Members of the DAPK family are generally involved in both apoptotic and autophagy pathways and share significant overall sequence similarity with myosin light chain-related kinases and triple functional domain protein-related kinases (Temmerman et al., 2013). DAPK1 and DAPK2 bind Ca2+/CaM through a closely related ARD, which is inhibited by phosphorylation of an identical ARD residue Ser308 in both kinases (Shani et al., 2001, Shohat et al., 2001). They also contain a basic loop (BL) in the kinase N lobe next to the kinase active site, which has been identified as a DAPK-family-specific signature motif (Tereshko et al., 2001). We found an identical type of dimer arrangement in all three kinases that involves the BL of the CD. In terms of functional implications, CD dimerization in hDAPK1, hDAPK2, and hDAPK3 is likely to inhibit catalytic activity by directly occluding the kinase active site.

To explore the molecular mechanisms involved in human DAPK regulation, we expressed and purified truncated versions of hDAPK1, hDAPK2, and hDAPK3. Both the hDAPK1 and hDAPK2 constructs encompass the CD and ARD segments. All three kinases were crystallized and the resulting structures were refined to a resolution of 2.0 Å (hDAPK1), 1.47 Å (hDAPK2), and 3.1 Å (hDAPK3). The hDAPK2 crystal contained two of these dimers per asymmetric unit, referred to as chains A/B and C/D, which provided an additional assessment of experimental error (details described in the legend). We addressed this question using hDAPK2, as its high-resolution structure provides the most accurate data on dimer interface interactions. The second main dimer interface is formed from positively charged residues on the DAPK signature BL segment, which belongs to the most mobile areas in the DAPK structures. In DAPK2, the main residues that contribute to the polar interactions are Arg47, Arg50, and Arg53 as well as the active-site residue Glu100 and Asp220 from the loop preceding helix αG. By contrast, in the DAPK2 structure, Glu182 is blocked by an interaction with Arg303 from the ARD, which acts as a pseudosubstrate. DAPK2 comprises an additional C-terminal tail segment that is predicted to be unstructured, and which has been shown to contribute to kinase activation via another dimerization mechanism that has not yet been fully characterized (Shani et al., 2001). The fitting procedure identified a mixture of 51% hDAPK2 monomer and 49% hDAPK2 dimer as the best solution (for details on software used see Supplemental Experimental Procedures). What hinders autonomous ARD-mediated Ca2+/CaM interactions in the absence of CD-mediated Ca2+/CaM binding at the molecular level is not yet fully understood. This could result from pseudosubstrate-type interactions of the N-terminal part of the ARD with the CD active-site area, as observed in various CD + ARD structures of members of the DAPK family, which may occlude the ARD segment from being accessible for Ca2+/CaM binding.

>[4x]GMEPFKQQKVEDFYDIGEELGSGQFAIVKKCREKSTGLEYAAKFIKKRQSRASRRGVSREEIEREVSILRQVLHHNVITLHDVYENRTDVVLILELVSGGELFDFLAQKESLSEEEATSFIKQILDGVNYLHTKKIAHFDLKPENIMLLDKNIPIPHIKLIDFGLAHEIEDGVEFKNIFGTPEFVAPEIVNYEPLGLEADMWSIGVITYILLSGASPFLGDTKQETLANITSVSYDFDEEFFSHTSELAKDFIRKLLVKETRKRLTIQEALRHPWITPVDNQQAMVRRESVVNLENFRKQYVRRRWKLSFSIVSLCNHLTR> MNITIYDVAREANVSMATVSRVVNGNPNVKPTTRKKVLEAIERL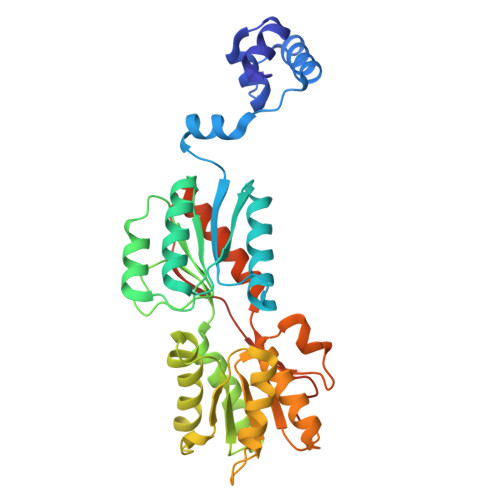GYRPNAVARGLASKKTTTVGVIIPDISSIFYSELARGIEDIATMYKYNIILSNSDQNMEKELHLLNTMLGKQVDGIVFMGGNITDEHVAEFKRSPVPIVLAASVEEQEETPSVAIDYEQAIYDAVKLLVDKGHTDIAFVSGPMAEPINRSKKLQGYKRALEEANLPFNEQFVAEGDYTYDSGLEALQHLMSLDKKPTAILSATDEMALGIIHAAQDQGLSIPEDLDIIGFDNTRLSLMVRPQLSTVVQPTYDIGAVAMRLLTKLMNKEPVEEHIVELPHRIELRKSTKSHHHHHH>MGHHHHHHSGENLYFQSGGMVAPTSNPGVPDELDGVPAVVDCDVHAVLPSPHSLIPYLDEYWADQLVAQLAPTYEPNYHPRGSAIAQHSDASVDENGRAATTAENLVKDVFADGFTDFAVVNCLYGVQQIHQPRREMAHARALNHWIANEWLDKDDRLRASIVVPQGSPRAAAEEIDFWSGDKRFVQVLLLGQSELLYGREINWPIWEAAEAAGLPVTLHIGGVFRQAPTSVGWPASHLEWYVGQQSNIEAQLNSIISEGILQKFPKTKILLSELGFNWLPPFMWKFDKLWKSYRPDIPWVQESPLELIREHVRVTTSPSDGAEEAGRLDSIVDRLGSDRMLVYSSDYPHKHHSGPRDIENGTHSPELLDRIYRRNAFDLYNLVVPSPGKVG[4x];>[4x]MTIIEHGSLGTLPAPSVTTGIVDADIHPVPQDGALEPYLDDRWKKHIREYGVRTTTGLQFISEYPQMYGGAMRADAWPESGYPGSDRELLRTQLLDKHNIQLGVLQCLAPGGQTLNPAGQALNQELAAALCRATNDWQLEHLVYPDPRMRAAIPVTFETPDYAVAEIERVGADPGVVAVLGTSKTLEPLGSRKYWPIYEASVAQNLPIQFHLSQGGGHANTGTGWTSYHTEYHTGHVQSFQSQLLSLVLSGTFDRFPTLKVMFVEGNVAHFAPLIQRMDYTWETLRGELPDLQRKPSEYIRDHIWASTQPIDEPEKPEHLAELLEEFCGDNVVFATDYPHFDFDDPETAFPRSFPVDLRDKILRGNGMRFFGVTNQAD

Here we report that the 2-aminoisobutyric acid hydroxylase from Rhodococcus wratislaviensis, AibH1H2, requires manganese to functionalize a strong, aliphatic C–H bond (BDE = 100 kcal/mol). Structural and spectroscopic studies of this enzyme reveal a redox-active, heterobimetallic manganese–iron active site at the locus of O2 activation and substrate coordination. Metabolism of 2-aminoisobutyric acid (AIB) in Rhodococcus wratislaviensis proceeds via the initial, selective hydroxylation of the pro-(R) methyl group by the monooxygenase AibH1H2 to furnish α-methyl-d-serine (d-MeSer). Previously, recombinant expression of AibH1H2 in Escherichia coli enabled its structural characterization and revealed distinct mono- and dinuclear metal binding sites housed within the AibH1 and AibH2 protein subunits, respectively.

We expressed AibH1H2 in E. coli grown in M9 minimal medium supplemented with excess FeII, and subsequent purification furnished protein samples (FeAibH1H2) containing ∼3 equiv of Fe per AibH1H2 heterodimer and minimal heterometal content (entry 1). Fe occupancy in both the mononuclear (Site 0) and dinuclear (Sites 1 and 2) metal sites was evident by inspection of the anomalous dispersion maps obtained from X-ray diffraction experiments performed on single crystals of FeAibH1H2. AibH1H2 had no detectable activity upon the exclusive incorporation of iron ions. Initial assays to determine the enzymatic activity were performed by mixing FeAibH1H2 with the AIB substrate and sodium ascorbate as a sacrificial reductant under aerobic conditions. Subsequent workup and gas chromatography–mass spectrometry (GC-MS) analyses of these solutions revealed minimal d-MeSer production. Since the protein structures of these two samples were found to be identical (RMSD = 0.34 Å over all atoms), our findings suggested an apparent requirement for one or more Mn ions in AibH1H2.>[2x]ADRNLRDLLAPWVPDAPSRALREMTLDSRVAAAGDLFVAVVGHQADGRRYIPQAIAQGVAAIIAEAKDEATDGEIREMHGVPVIYLSQLNERLSALAGRFYHEPSDNLRLVGVTGTNGK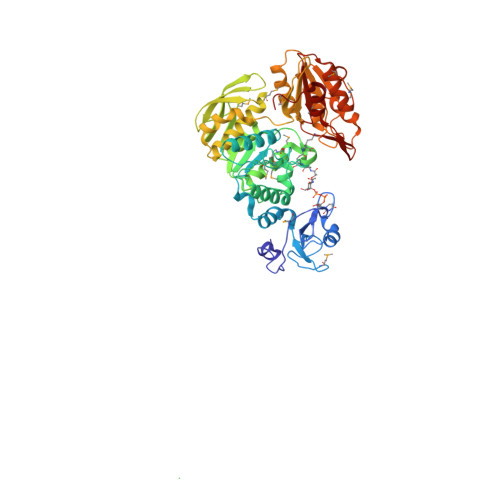TTTTQLLAQWSQLLGEISAVMGTVGNGLLGKVIPTENTTGSAVDVQHELAGLVDQGATFCAMEVSSHGLVQHRVAALKFAASVFTNLSRDHLDYHGDMEHYEAAKWLLYSEHHCGQAIINADDEVGRRWLAKLPDAVAVSMEDHINPNCHGRWLKATEVNYHDSGATIRFSSSWGDGEIESHLMGAFNVSNLLLALATLLALGYPLADLLKTAARLQPVCGRMEVFTAPGKPTVVVDYAHTPDALEKALQAARLHCAGKLWCVFGCGGDRDKGKRPLMGAIAEEFADVAVVTDDNPRTEEPRAIINDILAGMLDAGHAKVMEGRAEAVTCAVMQAKENDVVLVAGKGHEDYQIVGNQRLDYSDRVTVARLLGVIARSHH>MEPHVLGAGLYWLLLPCTLLAASLLRFNALSLVYLLFLLLLPWLPGPSRHSIPGHTGRLLRALLCLSLLFLVAHLAFQICLHTVPHLDQFLGQNGSLWVKVSQHIGVTRLDLKDIFNTTRLVAPDLGVLLASSLCLGLCGRLTRKAGQSRRTQELQDDDDDDDDDDEDIDAAPAVGLKGAPALATKRRLWLASRFRVTAHWLLMTSGRTLVIVLLALAGIAHPSAFSSIYLVVFLAICTWWSCHFPLSPLGFNTLCVMVSCFGAGHLICLYCYQTPFIQDMLPPGNIWARLFGLKNFVDLPNYSSPNALVLNTKHAWPIYVSPGILLLLYYTATSLLKLHKSCPSELRKETPREDEEHELELDHLEPEPQARDATQGEMPMTTEPDLDNCTVHVLTSQSPVRQRPVRPRLAELKEMSPLHGLGHLIMDQSYVCALIAMMVWSIMYHSWLTFVLLLWACLIWTVRSRHQLAMLCSPCILLYGLTLCCLRYVWAMELPELPTTLGPVSLHQLGLEHTRYPCLDLGAMLLYLLTFWLLLRQFVKEKLLKKQKVPAALLEVTVADTEPTQTQTLLRSLGELVTGIYVKYWIYVCAGMFIVVSFAGRLVVYKIVYMFLFLLCLTLFQVYYTLWRKLLRVFWWLVVAYTMLVLIAVYTFQFQDFPTYWRNLTGFTDEQLGDLGLEQFSVSELFSSILIPGFFLLACILQLHYFHRPFMQLTDLEHVPPPGTRHPRWAHRQDAVSEAPLLEHQEEEEVFREDGQSMDGPHQATQVPEGTASKWGLVADRLLDLAASFSAVLTRIQVFVRRLLELHVFKLVALYTVWVALKEVSVMNLLLVVLWAFALPYPRFRPMASCLSTVWTCIIIVCKMLYQLKIVNPHEYSSNCTEPFPNNTNLQPLEINQSLLYRGPVDPANWFGVRKGYPNLGYIQNHLQILLLLVFEAVVYRRQEHYRRQHQQAPLPAQAVCADGTRQRLDQDLLSCLKYFINFFFYKFGLEICFLMAVNVIGQRMNFMVILHGCWLVAILTRRRREAIARLWPNYCLFLTLFLLYQYLLCLGMPPALCIDYPWRWSKAIPMNSALIKWLYLPDFFRAPNSTNLISDFLLLLCASQQWQVFSAERTEEWQRMAGINTDHLEPLRGEPNPIPNFIHCRSYLDMLKVAVFRYLFWLVLVVVFVAGATRISIFGLGYLLACFYLLLFGTTLLQKDTRAQLVLWDCLILYNVTVIISKNMLSLLSCVFVEQMQSNFCWVIQLFSLVCTVKGYYDPKEMMTRDRDCLLPVEEAGIIWDSICFFFLLLQRRIFLSHYFLHVSADLKATALQASRGFALYNAANLKSINFHRQIEEKSLAQLKRQMKRIRAKQEKYRQSQASRGQLQSKDPQDPSQEPGPDSPGGSSPPRRQWWRPWLDHATVIHSGDYFLFESDSEEEEEALPEDPRPAAQSAFQMAYQAWVTNAQTVLRQRRERARQERAEQLASGGDLNPDVEPVDVPEDEMAGRSHMMQRVLSTMQFLWVLGQATVDGLTRWLRAFTKHHRTMSDVLCAERYLLTQELLRVGEVRRGVLDQLYVGEDEATLSGPVETRDGPSTASSGLGAEEPLSSMTDDTSSPLSTGYNTRSGSEEIVTDAGDLQAGTSLHGSQELLANARTRMRTASELLLDRRLHIPELEEAERFEAQQGRTLRLLRAGYQCVAAHSELLCYFIIILNHMVTASAASLVLPVLVFLWAMLTIPRPSKRFWMTAIVFTEVMVVTKYLFQFGFFPWNSYVVLRRYENKPYFPPRILGLEKTDSYIKYDLVQLMALFFHRSQLLCYGLWDHEEDRYPKDHCRSSVKDREAKEEPEAKLESQSETGTGHPKEPVLAGTPRDHIQGKGSIRSKDVIQDPPEDLKPRHTRHISIRFRRRKETPGPKGTAVMETEHEEGEGKETTERKRPRHTQEKSKFRERMKAAGRRLQSFCVSLAQS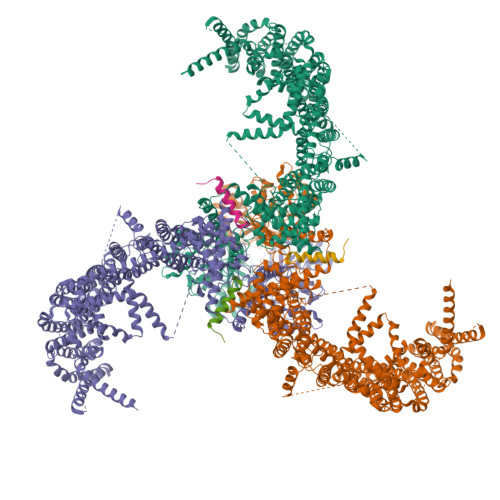FYQPLQRFFHDILHTKYRAATDVYALMFLADIVDIIIIIFGFWAFGKHSAATDIASSLSDDQVPQAFLFMLLVQFGTMVIDRALYLRKTVLGKLAFQVVLVVAIHIWMFFILPAVTERMFSQNAVAQLWYFVKCIYFALSAYQIRCGYPTRILGNFLTKKYNHLNLFLFQGFRLVPFLVELRAVMDWVWTDTTLSLSNWMCVEDIYANIFIIKCSRETEKKYPQPKGQKKKKIVKYGMGGLIILFLIAIIWFPLLFMSLIRSVVGVVNQPIDVTVTLKLGGYEPLFTMSAQQPSIVPFTPQAYEELSQQFDPYPLAMQFISQYSPEDIVTAQIEGSSGALWRISPPSRAQMKQELYNGTADITLRFTWNFQRDLAKGGTVEYTNEKHTLELAPNSTARRQLAQLLEGRPDQSVVIPHLFPKYIRAPNGPEANPVKQLQPDEEEDYLGVRIQLRREQVGTGASGEQAGTKASDFLEWWVIELQDCKADCNLLPMVIFSDKVSPPSLGFLAGYGIVGLYVSIVLVVGKFVRGFFSEISHSIMFEELPCVDRILKLCQDIFLVRETRELELEEELYAKLIFLYRSPETMIKWTRERE[3x];>MSCAGEALAPGPAEQQCPVEAGGGRLGSPAHEACNEDNTEKDKRPATSGHTRCGLMRDQSIWPNPSAGELVRTQPERLPQLQTSAQEPGKEETGKIKNGGHTRMSNGNGIPHGAKHVSVENHKISAPVSQKMHRKIQSSLSVNNDISKKSKVNAVFSPKAASSPEDCCVHCILACLFCEFLTLCNIVLGQASCGICTSEACCCCCGDEMGDDCSCPCDMDCGIMDACCESSDCLEICMECCGICFPS[3x]>MASWSHPQFEKGAMQIRADFDSGNIQVIDASDPRRIRLAIRPDLASQHFQWFHFKVEGMAPATEHCFTLVNAGQSAYSHAWSGYQAVASYDGERWFRVPSQYDADGLHFQLEPEESEVRFAYFEPYSRERHARLVERALGIEGVERLAVGTSVQGRDIELLRVRRHPDSHLKLWVIAQQHPGEHMAEWFMEGLIERLQRPDDTEMQRLLEKADLYLVPNMNPDGAFHGNLRTNAAGQDLNRAWLEPSAERSPEVWFVQQEMKRHGVDLFLDIHGDEEIPHVFAAGCEGNPGYTPRLERLEQRFREELMARGEFQIRHGYPRSAPGQANLALACNFVGQTYDCLAFTIEMPFKDHDDNPEPGTGWSGARSKRLGQDVLSTLAVLVD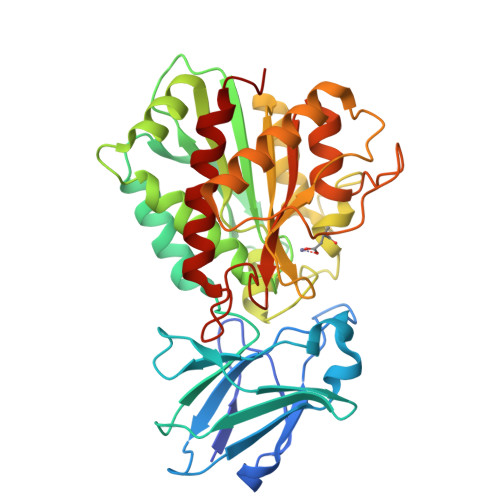ELR[2x]> GPMTSQKLVRLPGLIDVHVHLREPGGTHKEDFASGTAAALAGGITMVCAMPNTRPPIIDAPALALAQKLAEAGARCDFALFLGASSENAGTLGTVAGSAAGLKLYLANATTNSSHGVTSVVQWMEHFETWPSHLPIVAHAEQQTVAAVLMVAQLTQRSVHICHVARKEEILLIKAAKARGLPVTCEVAPHHLFLSHDDLERLGPGKGEVRPELGSRQDVEALWENMAVIDCFASDHAPHTLEEKCGSRPPPGFPGLETMLPLLLTAVSEGRLSLDDLLQRLHHNPRRIFHLPPQEDTYVEVDLEHEWTIPSHMPFSKAHWTPFEGQKVKGTVRRVVLRGEVAYI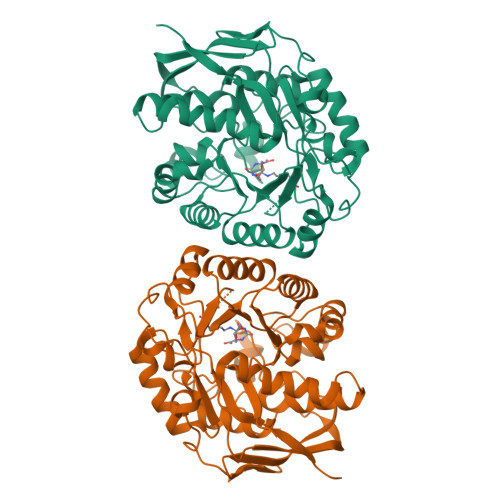DGQVLVPPGYGQDVRKWPQGAVPQLPP>[2x]MDRRSFITKAAVGGAAASALAAPALAQSAPKVTWRLASSFPKSLDTIFGGAEVLSKMLSEATDGNFQIQVFSAGELVPGLQAADAVTEGTVECCHTVGYYYWGKDPTFALAAAVPFSLSARGINAWHYHGGGIDLYNEFLSQHNIVAFPGGNTGVQMGGWFRREINTVADMQGLKMRVGGFAGK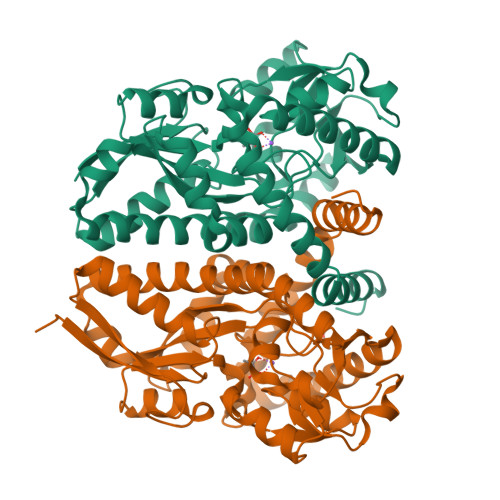VMERLGVVPQQIAGGDIYPALEKGTIDATEWVGPYDDEKLGFFKVAPYYYYPGWWEGGPTVHFMFNKSAYEGLTPTYQSLLRTACHAADANMLQLYDWKNPTAIKSLVAQGTQLRPFSPEILQACFEAANEVYAEMEASNPAFKKIWDSIKAFRSEHYTWAQIAEYNYDTFMMVQQNAGKL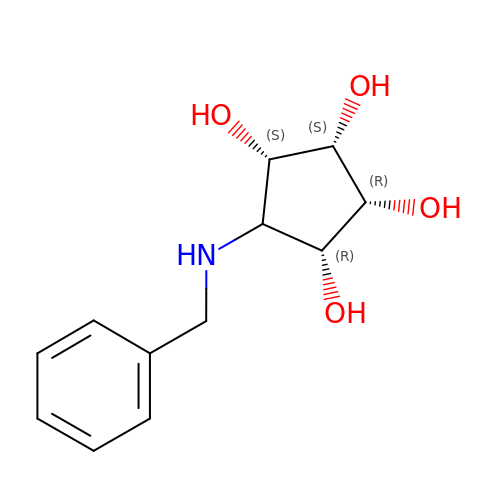(1R,2R,3S,4S,5R)-5-(BENZYLAMINO)CYCLOPENTANE-1,2,3,4-TETROL | C12 H17 N O4 | AQARFUBRAYWQBH-NMZKHRHQSA-N>MQNVLIVGVGFMGGSFAKSLRRSGFKGKIYGYDINPESISKAVDLGIIDEGTTSIAKVEDFS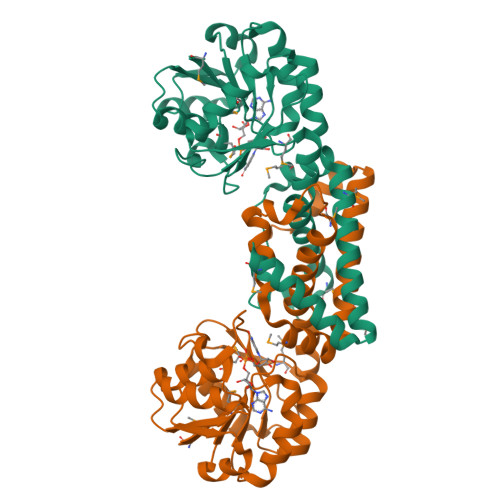PDFVMLSSPVRTFREIAKKLSYILSEDATVTDQGSVKGKLVYDLENILGKRFVGGHPIAGTEKSGVEYSLDNLYEGKKVILTPTKKTDKKRLKLVKRVWEDVGGVVEYMSPELHDYVFGVVSHLPHAVAFALVDTLIHMSTPEVDLFKYPGGGFKDFTRIAKSDPIMWRDIFLENKENVMKAIEGFEKSLNHLKELIVREAEEELVEYLKEVKIKRMEI[4x]VhChiP is a chitooligosaccharide-specific porin identified in the outer membrane of Vibrio campbellii type strain American Type Culture Collection BAA 1116. VhChiP contains three identical subunits, and in each subunit, the 19-amino acid N-terminal segment serves as a molecular plug (the “N-plug”) that controls the closed/open dynamics of the neighboring pores. VhChiP is a sugar-specific OM porin with the ability to selectively transport a range of chitooligosaccharides, chitohexaose being the most preferred. VhChiP consists of three identical β-barrels, each containing 16 β-strands connected on the extracellular side by eight hydrophilic loops and on the periplasmic side by eight short hydrophobic turns.

X-ray diffraction data from truncated VhChiP cocrystallized with chitohexaose were obtained to a resolution of 2.75 Å. The data were processed in the triclinic P1 space group with two trimers per asymmetric unit. We observed electron density for the sugar ligand in all six protein chains (two trimeric molecules). However, the complete electron density map of six GlcNAc rings of chitohexaose was observed only in chains B and F, while the electron densities of the sugar molecules in chains A, C, D, and E were partial, missing mainly the areas assigned to GlcNAc-1 (nonreducing end) and GlcNAc-6 (reducing end) of the sugar chain. For the structures of chains B and F,, the sugar chain was fully extended inside the pore, in a similar manner to chitohexaose found in the native structure. We observed that each of the trimeric β-barrels contained one molecule of chitohexaose inside the channel lumen in which the reducing end sugar (GlcNAc-1) made π–π interactions with the plane of the aromatic side chains of Trp123 and Tyr349. At affinity site 2, two weak hydrogen bonds were observed, one between the carboxylate side chains of Asp127 and the O-acetamido group of GlcNAc-2 (3.02 Å) and another between the side chain of Glu347 and the N-acetamido group of GlcNAc-2 (3.24 Å). For affinity sites 3 and 4, only one hydrogen bond was seen at each site, in which the carboxyl side chain of Asp122 bonded with the N-acetamido group of GlcNAc-3 (3.00 Å) and of Glu53 with the N-acetamido group of GlcNAc-4 (3.17 Å). Five hydrogen bonds were missing in the truncated structure (residues highlighted in green), including the N-acetamido group of GlcNAc-2/Arg312 (2.95 Å) and GlcNAc-3/Arg94 (2.91 Å), the O-acetamido groups of GlcNAc-3/Arg148 (2.96 Å) and Glu53/O-acetamido of GlcNAc-3 (2.95 Å), the O-acetamido of GlcNAc-3 Arg312/O- (2.90 Å) and the O-acetamido of GlcNAc-4/Asp135 (2.96 Å)/Asp145 (2.95 Å). Structural analysis of sugar–channel interactions suggested that N-plug deletion led to the loss of five hydrogen bonds that interacted with the GlcNAc moieties at the central affinity site, thus drastically weakening the binding affinity of the truncated channel.

>[6x]EVYGIIAMQAAYRDYDSGDAKQDDNLGGMQLNNESRIGFRGKKQFANFEPTFIWQIEGGYVDPSFGGEGAGLGERDTFVGFESASWGQVRLGRVLTPMYELVDWPASNPGLGDVYDWGGAIGGAKYQDRQSNTIRWDSPMYADKFSIDAAVGAGDKAGLGAGDDYWGGIAAHYKLGPLQLDAAYEGNRNIEAEGQTWENNTYLVGVQGWFENGISFFAQYKYMEADASNGVNEKQDAMSAGLMYTTGDWQYKLGYAANFDLERDGKTLSNTSDDVVSAQIMYFVDPSAVLYARARMNDFNEGLDGLDDAARWTSGTNGDYNEYSVGVEYYF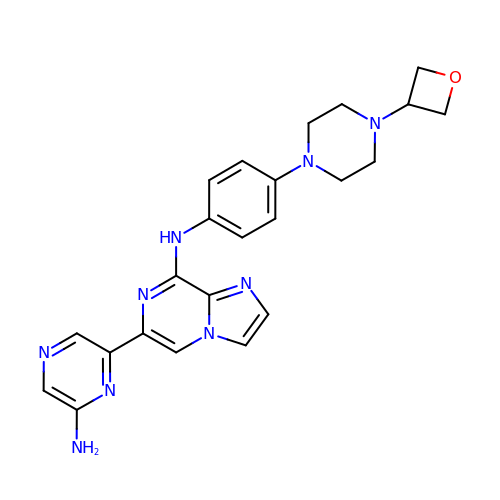6-(6-aminopyrazin-2-yl)-N-{4-[4-(oxetan-3-yl)piperazin-1-yl]phenyl}imidazo[1,2-a]pyrazin-8-amine | C23 H25 N9 O | XCIGZBVOUQVIPI-UHFFFAOYSA-N Pitavastatin | C25 H24 F N O4 | 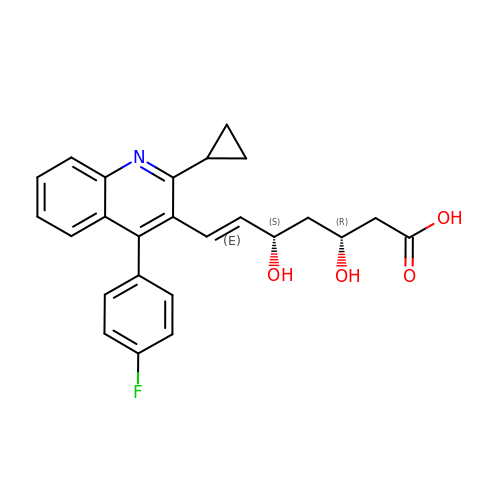VGYFMXBACGZSIL-MCBHFWOFSA-N> NSVSMIGKIAETDVSG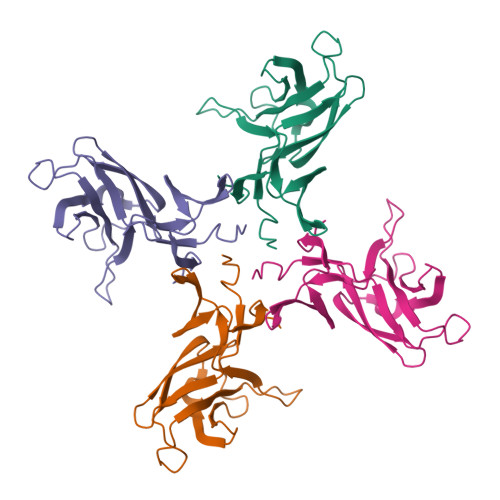ANFDGNNKLSFSLFFDEKIDASKGVPAIQILNENNELVKTIPLKDYNGQKGYINFEWDGTNEKGEKVPKGNYKIKAEYNLDSHSKQYLQTRIGRGEVESVIFDKGKPMLRMGEMVLPIDSAIEFYQPDQK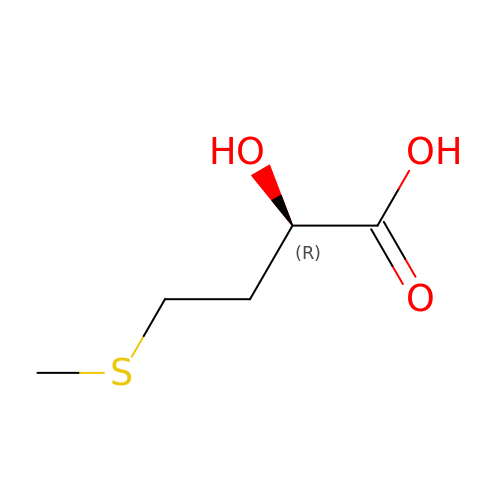4-methylsulfanyl-2-oxidanyl-butanoic acid | C5 H10 O3 S | ONFOSYPQQXJWGS-UHFFFAOYSA-N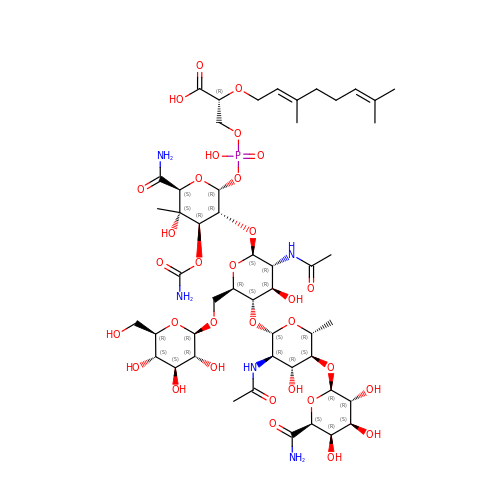(2R)-3-{[(S)-{[(2R,3R,4R,5S,6S)-3-{[(2S,3R,4R,5S,6R)-3-(acetylamino)-5-{[(2S,3R,4R,5S,6R)-3-(acetylamino)-5-{[(2R,3R,4S,5R,6S)-6-carbamoyl-3,4,5-trihydroxytetrahydro-2H-pyran-2-yl]oxy}-4-hydroxy-6-methyltetrahydro-2H-pyran-2-yl]oxy}-4-hydroxy-6-({[(2R,3R,4S,5S,6R)-3,4,5-trihydroxy-6-(hydroxymethyl)tetrahydro-2H-pyran-2-yl]oxy}methyl)tetrahydro-2H-pyran-2-yl]oxy}-6-carbamoyl-4-(carbamoyloxy)-5-hydroxy-5-methyltetrahydro-2H-pyran-2-yl]oxy}(hydroxy)phosphoryl]oxy}-2-{[(2Z)-3,7-dimethylocta-2,6-dien-1-yl]oxy}propanoic acid | C49 H80 N5 O32 P | RAPYBPXXZJZLIC-LMVGRRJQSA-N>GDHGPEFNGVMVVKAAEAEELPDDLMNFKGTWEVSADGSSGRFFSKGATDSYVFHLIPAKDVKKPGWREHNEVKDSYIKIDKQSIAARYKTSTTAPYSVAFKVNTKSLIKDHDYKITFEQGQIASGITVDYRIGSAFNKTTDDSFKISDESKYASNVKIEGEEQGFKQREQGDKTISFRTLKEGPMSLVLLSKVEKKPQGDLDVEFKNLKIIDVTNPSQLDKGVAYVGNKNVQLTLKSDDGRTNFEGDEISLFNSRGELLQTVTVTKDQQNPISITLSEDQAKSLKNKEKLKVSIKQKQSKKTSKDFFF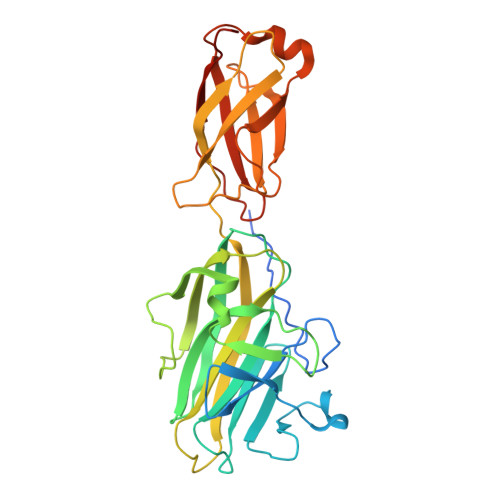EVGIDPKVEAK[4x]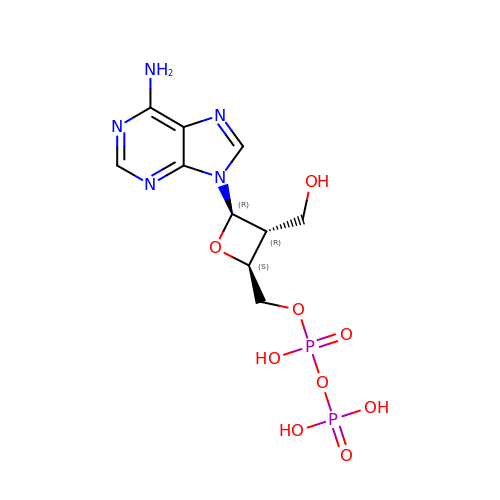[(2S,3R,4R)-4-(6-amino-9H-purin-9-yl)-3-(hydroxymethyl)oxetan-2-yl]methyl trihydrogen diphosphate | C10 H15 N5 O9 P2 | HJOFGDMHIXEUNX-OXOINMOOSA-N>[2x]MHHHHHHSTSVDLGTENLYFQSNAEERAAGARPSATQTTGTATEPFHGPHQAGIATPPQAHAVFLGLDLRKGTGRKELGRLMRLLTDDARRLTQGRPALADPEPDLAPLPSRLTFTFGFGPGLFKAAGLEKQRPEGLRPLPPFKVDRLEDRWSGGDLLVQICCDDPITLAHALRMTVKDARAFTRVRWVQRGFRRSPGVQSSGATQRNLMGQLDGTVNPVPGTADFDQAVWVQDGPEWLR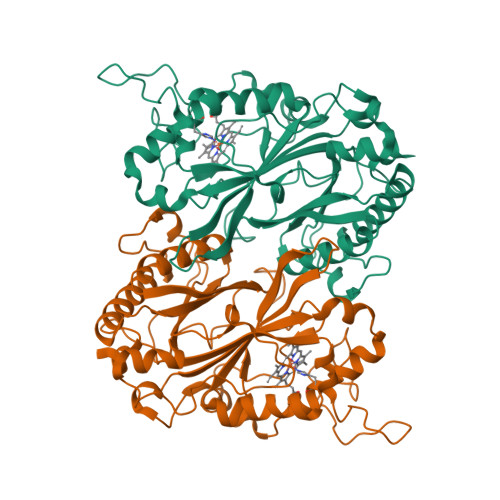GGTTLVLRRIRMELEKWDEADPAGKEFAVGRRLTSGAPLTGRHEHDEPDFDAVDSAGFPVIAENAHIRLAHVDSPRLRMLRRPYNYDEGLTADGRSDAGLLFAAYQADIDRQFIPVQRRLDEGGDLLNLWTTPIGSAVFAIPPGCDENGWIGQGLLG>[2x]MHDEREGYLEILSRITTEEEFFSLVLEICGNYGFEFFSFGARAPFPLTAPKY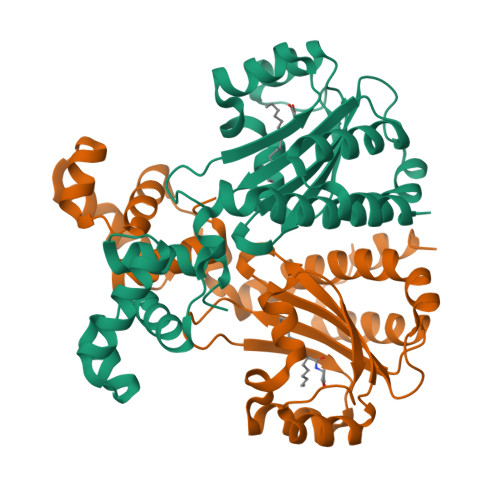HFLSNYPGEWKSRYISEDYTSIDPIVRHGLLEYTPLIWNGEDFQENRFFWEEALHHGIRHGWSIPVRGKYGLISMLSLVRSSESIAATEILEKESFLLWITSMLQATFGDLLAPRIVPESNVRLTARETEMLKWTAVGKTYGEIGLILSIDQRTVKFHIVNAMRKLNSSNKAEATMKAYAIGLLN>MLTMKDIIRDGHPTLRQKAAELELPLTKEEKETLIAMREFLVNSQDEEIAKRYGLRSGVGLAAPQINISKRMIAVLIPDDGSGKSYDYMLVNPKIVSHSVQEAYLPTGEGCLSVDDNVAGLVHRHNRITIK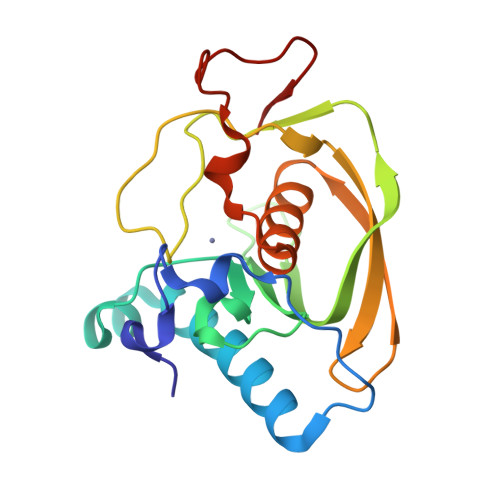AKDIEGNDIQLRLKGYPAIVFQHEIDHLNGVMFYDHIDKNHPLQPHTDAVEV[2x]>MTVEPFRNEPIETFQTEEARRAMREALRRVREEFGRHYPLYIGGEWVDTKERM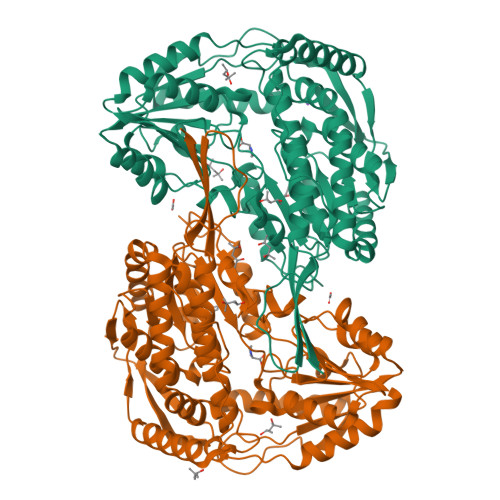VSLNPSAPSEVVGTTAKAGKAEAEAALEAAWKAFKTWKDWPQEDRSRLLLKAAALMRRRKRELEATLVYEVGKNWVEASADVAEAIDFIEYYARAALRYRYPAVEVVPYPGEDNESFYVPLGAGVVIAPWNFPVAIFTGMIVGPVAVGNTVIAKPAEDAVVVGAKVFEIFHEAGFPPGVVNFLPGVGEEVGAYLVEHPRIRFINFTGSLEVGLKIYEAAGRLAPGQTWFKRAYVETGGKNAIIVDETADFDLAAEGVVVSAYGFQGQKCSAASRLILTQGAYEPVLERVLKRAERLSVGPAEENPDLGPVVSAEQERKVLSYIEIGKNEGQLVLGGKRLEGEGYFIAPTVFTEVPPKARIAQEEIFGPVLSVIRVKDFAEALEVANDTPYGLTGGVYSRKREHLEWARREFHVGNLYFNRKITGALVGVQPFGGFKLSGTNAKTGALDYLRLFLEMKAVAERF[2x]The membrane-bound protein EssC is an integral component of the bacterial Type VII secretion system (T7SS), which is a determinant of virulence in important Gram-positive pathogens. The protein is predicted to consist of an intracellular repeat of forkhead-associated (FHA) domains at the N-terminus, two transmembrane helices and three P-loop-containing ATPase-type domains, D1–D3, forming the C-terminal intracellular segment. We present crystal structures of the N-terminal FHA domains (EssC-N) and a C-terminal fragment EssC-C from Geobacillus thermodenitrificans, encompassing two of the ATPase-type modules, D2 and D3. The observation of protomer contacts in the crystal structure of EssC-C together with similarity to the DNA translocase FtsK, suggests a model for a hexameric EssC assembly.

EssC-N consists of residues Met1–Leu195 folded into a two-domain structure with each domain representative of the β-sandwich FHA fold. Residues Met1–Glu91 constitute domain FHA1, which is linked to FHA2 via a short dipeptide linker (Glu92 and Gln93). FHA1 and FHA2 domains consist of nine and 12 β-strands respectively with the domains aligned almost perpendicular to each other. The domain–domain contacts are mainly via van der Waals interactions between side chains. A pronounced feature at the domain–domain interface is Trp5 nestled into a cavity formed by Leu162, Pro164 and Tyr165. Hydrogen-bonding interactions also contribute to the domain alignments, with a network of three glutamines (residues 3, 93, and 167) and a water molecule interacting at one end of the interface. Seven residues are missing from the model of FHA1 due to insufficient electron density. These residues (at positions 19, 20, 53, 54, 80, 81 and 82) are located on turns linking β-strands. However, as reported by Tanaka et al., motifs common to many FHA domains and residues implicated in the recognition and binding of phosphothreonine, as exemplified by Ki67 are absent from EssC-N.

> MSQLWVLYETYCQLFSLTNEEKVIVIGNQLEHHVTVSSFSFRNGYIQIEKKSDGSTLAVLQGGRQIGELKPRCSITIDVDGQQMTIAWSGEEQRKYVYYVGQQSEVLVSNDPQADIETTNARFSLRKHRGQWVVIPDDDAPLFLNGVQLSDAVSLRNGDVLLCPYMQFVFIEEDLLAVTSSEEVVSSLTETMPPLS> MADVPAGVTLAEKQTLVRNNGSEVQSLDPHKIEGVPESNISRDLFEGLLVSDLDGHPAPGVAESWDNKDAKVWTFHLRKDAKWSDGTPVTAQDFVYSWQRSVDPNTASPYASYLQYGHIAGIDEILEGKKPITDLGVKAIDDHTLEVTLSEPVPYFYKLLVHPSTSPVPKAAIEKFGEKWTQPGNIVTNGAYTLKDWVVNERIVLERSPTYWNNAKTVINQVTYLPIASEVTDVNRYRSGEIDMTNNSMPIELFQKLKKEIPDEVHVDPYLCTYYYEINNQKPPFNDVRVRTALK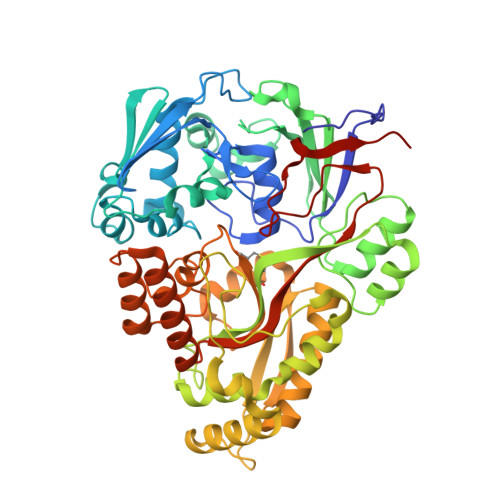LGMDRDIIVNKVKAQGNMPAYGYTPPYTDGAKLTQPEWFGWSQEKRNEEAKKLLAEAGYTADKPLTINLLYNTSDLHKKLAIAASSLWKKNIGVNVKLVNQEWKTFLDTRHQGTFDVARAGWCADYNEPTSFLNTMLSNSSMNTAHYKSPAFDSIMAETLKVTDEAQRTALYTKAEQQLDKDSAIVPVYYYVNARLVKPWVGGYTGKDPLDNTYTRNMYIVKHHHHHHH>MSHHHHHHSSGLEVLFQGPMAEKQKHDGRVKIGHYVLGDTLGVGTFGKVKIGEHQLTGHKVAVKILNRQKIRSLDVVGKIKREIQNLKLFRHPHIIKLYQVISTPTDFFMVMEYVSGGELFDYICKHGRVEEMEARRLFQQILSAVDYCHRHMVVHRDLKPENVLLDAHMNAKIADFGLSNMMSDGEFLRTSCGSPNYAAPEVISGRLYAGPEVDIWSCGVILYALLCGTLPFDDEHVPTLFKKIRGGVFYIPEYLNRSVATLLMHMLQVDPLKRATIKDIREHEWFKQDLPSYLFPEDPSYDANVIDDEAVKEVCEKFECTESEVMNSLYSGDPQDQLAVAYHLIIDNRRIMNQASEFYLASSPPSGSFMDDSAMHIPPGLKPHPERMPPLIADSPKARCPLDALNTTKPKSLAVKKAKWHLGIRSQSKPYDIMAEVYRAMKQLDFEWKVVNAYHLRVRRKNPVTGNYVKMSLQLYLVDNRSYLLDFKSIDDEVVEQRSGSSTPQRSCSAAGLHRPRSSFDSTTAESHSLSGSLTGSLTGSTLSSVSPRLGSHTMDFFEMCASLITTLAR[2x];>[2x]MGLNDIFEAQKIEWHEMGNTSSERAALERHGGHKTPRRDSSGGTKDGDRPKILMDSPEDADLFHSEEIKAPEKEEFLAWQHDLEVNDKAPAQARPTVFRWTGGGKEVYLSGSFNNWSKLPLTRSHNNFVAILDLPEGEHQYKFFVDGQWTHDPSEPIVTSQLGTVNNIIQVKKTDFEVFDALMVDSQKCSDVSELSSSPPGPYHQEPYVCKPEERFRAPPILPPHLLQVILNKDTGISCDPALLPEPNHVMLNHLYALSIKDGVMVLSATHRYKKKYVTTLLYKPI;>METVISSDSSPAVENEHPQETPESNNSVYTSFMKSHRCYDLIPTSSKLVVFDTSLQVKKAFFALVTNGVRAAPLWDSKKQSFVGMLTITDFINILHRYYKSALVQIYELEEHKIETWREVYLQDSFKPLVCISPNASLFDAVSSLIRNKIHRLPVIDPESGNTLYILTHKRILKFLKLFITEFPKPEFMSKSLEELQIGTYANIAMVRTTTPVYVALGIFVQHRVSALPVVDEKGRVVDIYSKFDVINLAAEKTYNNLDVSVTKALQHRSHYFEGVLKCYLHETLETIINRLVEAEVHRLVVVDENDVVKGIVSLSDILQALVLTGGEKKP[2x]

AMP-activated protein kinase (AMPK) plays an important role in regulating energy homeostasis in eukaryotic cells. AMPK is a heterotrimeric enzyme complex composed of a catalytic α-subunit, together with β- and γ-regulatory subunits. The α-subunit contains an N-terminal protein kinase domain and a C-terminal regulatory domain. The γ-subunit contains four copies of a cystathionine-β-synthase domain27, and we previously showed that the γ-subunit binds three molecules of adenine nucleotide.

In our new structure, the CBM is ordered and bound to the N-terminal lobe of the kinase domain. The interface between these two domains generates the binding cavity for 991. One end of the five stranded β-sheet that constitutes the core of the N-terminal domain of the kinase packs against a pair of anti-parallel β-strands from the CBM. 991 sits in a pocket generated at this interface and interacts with hydrophobic residues from each domain, mainly involving ring-1 and ring-2 of the activator. Interestingly, the phosphorylated serine (pSer) at position 108 from the CBM is involved in a network of electrostatic interactions with Lys-31(Kinase) and potentially Thr-21(Kinase) and Asn-111(CBM). Mutations of Lys-29(Kinase)/Lys-31(Kinase), Arg-83(CBM) and Ser-108(CBM) all lead to more than a 25-fold reduction in activator affinity, without altering the regulation of AMPK by AMP. An α-helix immediately C-terminal to the CBM, absent in previous crystal structures of the CBM38 and just outside of the CBM consensus sequence, interacts with the αC helix of the kinase (hereafter, the C-interacting helix). However, the top of the C-helix is rotated away from the active site, relative to our earlier structure, such that the Lys-45->Glu-64 interaction is broken (which is regarded as essential for efficient phosphoryl transfer). Thus, by promoting this CBM/Kinase/regulatory–fragment interaction, 991 and A-769662 enhance protection of the activation loop against dephosphorylation.> DPSSRSTRKAVIGYYFIPTNQINNYTETDTSVVPFPVSNITPAKAKQLTHINFSFLDINSNLECAWDPATNDAKARDVVNRLTALKAHNPSLRIMFSIGGWYYSNDLGVSHANYVNAVKTPAARTKFAQSCVRIMKDYGFDGVDIDWEYPQAAEVDGFIAALQEIRTLLNQQTIADGRQALPYQLTIAGAGGAFFLSRYYSKLAQIVAPLDYINLMTYDLAGPWEKITNHQAALFGDAAGPTFYNALREANLGWSWEELTRAFPSPFSLTVDAAVQQHLMMEGVPSAKIVMGVPFYGRAFKGVSGGNGGQYSSHSTPGEDPYPNADYWLVGCDECVRDKDPRIASYRQLEQMLQGNYGYQRLWNDKTKTPYLYHAQNGLFVTYDDAESFKYKAKYIKQQQLGGVMFWHLGQDNR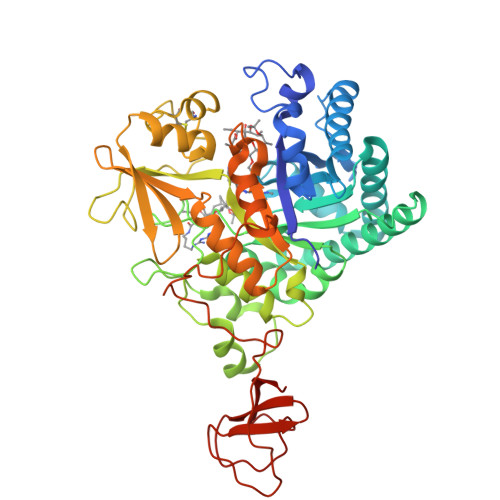NGDLLAALDRYFNAADYDDSQLDMGTGLRYTGVGPGNLPIMTAPAYVPGTTYAQGALVSYQGYVWQTKWGYITSAPGSDSAWLKVGRLA Indeed, URH1p was initially classified as a nucleoside hydrolase (NH) with a pronounced preference for uridine substrate but was later shown to also participate in a Preiss-Handler-dependent pathway for recycling of both endogenous and exogenous nicotinamide riboside (NR) towards NAD+ synthesis. We show that the URH1p has similar catalytic efficiencies for hydrolysis of NR and uridine, advocating a dual role of the enzyme in both NAD+ synthesis and nucleobase salvage. The crystal structure of URH1p showed that the enzyme belongs to the group I structural homology group of the Ca2+-dependent NHs and displays a monomeric structure that is unprecedented in this class of enzymes. The yeast URH1p, a cytosolic enzyme, was found to exhibit uridine and NR hydrolase activity, contributing both to the cell’s ability to recover uracil for nucleotide biosynthesis and maintain a balanced pool of nucleotides for DNA, RNA and cofactor synthesis and to regulate NAD+ concentration through the Preiss-Handler shunt.

The asymmetric unit of the hexagonal crystals contains two URH1p monomers, covalently linked by a disulphide bridge involving residue Cys142 from both chains. Making only marginal non-covalent interactions between the two protein monomers in the asymmetric unit, it is thus evident that the URH1p dimer found in the crystal is principally caused by an adventitious disulphide bridge between Cys142 residues, not representing a physiologically relevant quaternary arrangement. The URH1p structure retains the characteristic open (α, β) NH fold that is composed of an eight-stranded central mixed β-sheet (β1-β7 and β10) surrounded by the connecting α-helices, a helical domain that completes the active site, and two additional antiparallel β-strands (β8 and β9) extending away from the core sheet. The crystal structure of URH1p closely resembles the “closed” conformation observed for the ligand-bound NHs, with an ordered loop that connects strand β3 to helices α3.1 and α3.2 (the so-called “β3-α3 loop”) and a defined conformation of the α8 helix with only its short C-terminal portion (amino acids 242 to 246) flexible, as judged by the weak electron density. Since ligand-free group I NHs typically display high flexibility in the β3-α3 loop and α8 helix, we infer that the contacts with the Tris molecule found in the active site stabilise the observed closed conformation. Indeed, the side chain imidazole ring of His86, a crucial residue in modulating NH activity and structural dynamics, is within hydrogen bonding distance from one hydroxyl of the Tris molecule, and this interaction is likely pivotal for the closed conformation of the β3-α3 loop. Further contacts are observed between the Tris molecule and amino acid residues Asn42, Thr130, Asn165, Glu173, Asn175 and Asp255, whose homologues are involved in substrate binding in other NHs.

>[2x]GSHMTVSKIPIWLDCDPGHDDAIAILLGCFHPAFNLLGISTCFGNAPPENTDYNARSLLTAMGKAQAIPVYKGAQRPWKREPHYAPDIHGISGLDGTSLLPKPTFEARTDKTYIEAIEEAILANNGEISFVSTGALTTLATVFRCKPYLKKSVKYISIMGGGLHGLGNCNPNLSAEFNVWIDPDAANYIFRDPDVKDKCIVVPLNLTHKAIATYKVNEMIYNEKNNSKLRELFLELFQFFAHTYKDMQGFESGPPIHDPVASMPLLEFYGWDPSSAVGFRYKRMDISCIDDVFNENSGKIIIEKEYPNDSDVGTIIGLDLNIQYFWDQIFEALNRADKMSTIG>QMNYEEVIKKYRGEENFDHAAYDWRLHSGVTPVKDQKNCGSCWAFSSIGSVESQYAIRKNKLITLSEQELVDCSFKNYGCNGGLINNAFEDMIELGGICPDGDYPYVSDAPNLCNIDRCTEKYGIKNYLSVPDNKLKEALRFLGPISISVAVSDDFAFYKEGIFDGECGDQLNHAV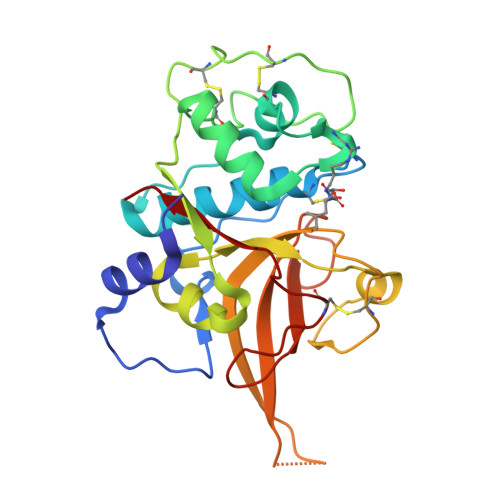MLVGFGMKEIVNPLTKKGEKHYYYIIKNSWGQQWGERGFINIETDESGLMRKCGLGTDAFIPLIE[4x]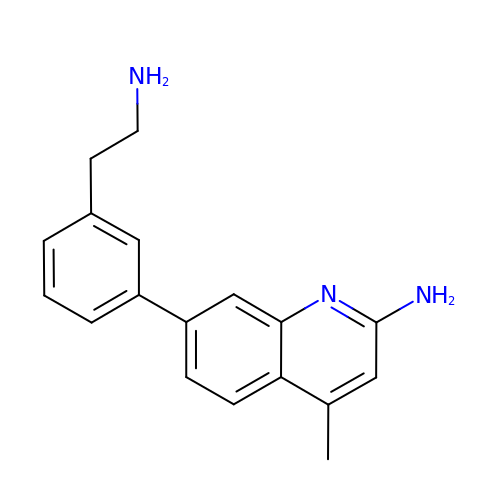7-[3-(2-aminoethyl)phenyl]-4-methylquinolin-2-amine | C18 H19 N3 | KEWLPOCHRHJHLA-UHFFFAOYSA-N>GAGCCTACCCTGTACGGACATCAG[3x];> TACACCGTACACCGTACACCG;>TCCTGATGTGGCTAGGC[3x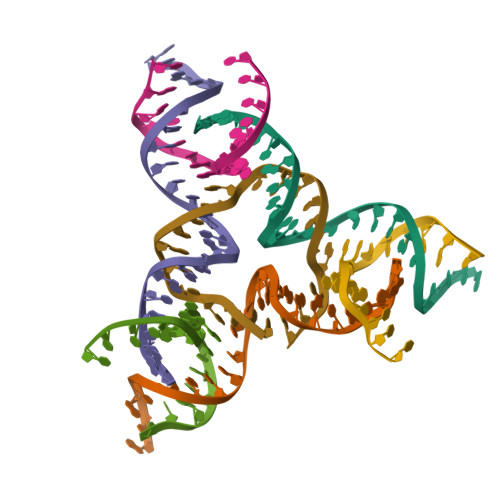]N-({3-[5-hydroxy-4-(7H-pyrrolo[2,3-d]pyrimidin-6-yl)-1H-pyrazol-1-yl]phenyl}methyl)-N'-phenylurea | C23 H19 N7 O2 | 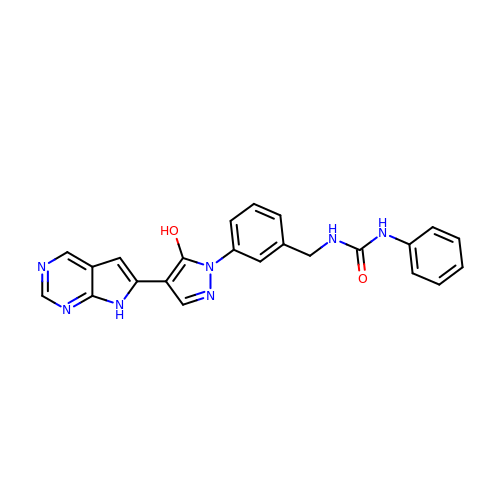QBPBWCKGIYYDOU-UHFFFAOYSA-N>[2x]GKDEIQIVDQDTSWQMDNKYIEEDIREQLGIDPFTDLVYLGYYGNPYTQLEAINDLVNTTLVGKNELSFKVKVTKPYKEDIKVNLMKEDKLVTDFPEMAEGIPLFPSENCTFEGGVLKAGELETTVKLTLKDVEKLNNLSGYVMAIKLTMEGSHEHLAIARTRSSYFVKLNLSIRLDNIDSSNKKIEGKGFNKEIS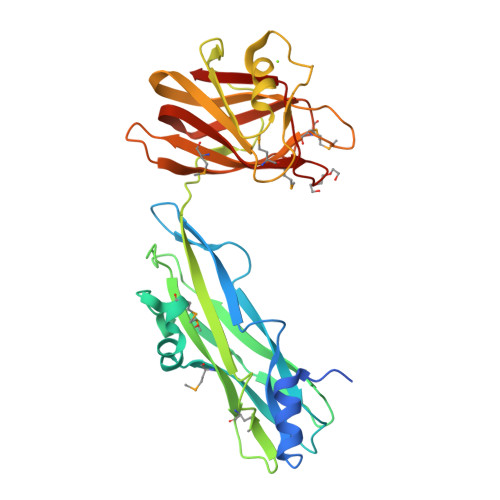FKSDIRPDKLGSLNDGNFTANNWYTSNANNYLTIILPEKQSLKGFRLDTNTSPSGSYMLKSCRVMVETPDGNWVNHGVFDRKSMDGIAYISFKKPVECTKVRFENMMAFNGRFSVDVNEVTAFR(2R)-2-(6-methoxynaphthalen-2-yl)propanoic acid 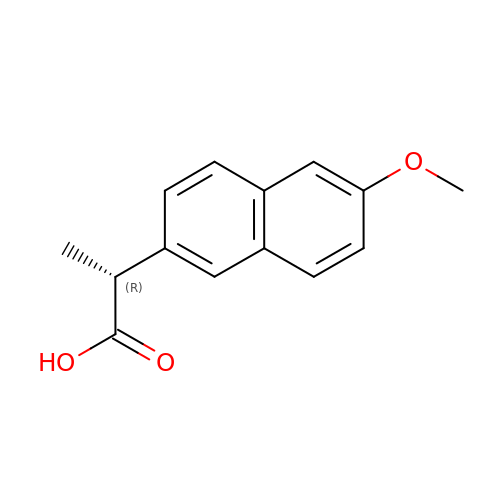| C14 H14 O3 | CMWTZPSULFXXJA-SECBINFHSA-N>MASQPNSSAKKKEEKGKNIQVVVRCRPFNLAERKASAHSIVECDPVRKEVSVRTGGLADKSSRKTYTFDMVFGASTKQIDVYRSVVCPILDEVIMGYNCTIFAYGQTGTGKTFTMEGERSPNEEYTWEEDPLAGIIPRTLHQIFEKLTDNGTEFSVKVSLLSIYNEELFDLLNPSSDVSERLQMFDDPRNKRGVIIKGLEEITVHNKDEVYQILEKGAAKRTTAATLMNAYSSRSHSVFSVTIHMKETTIDGEELVKIGKLNLVDLAGSENIGRSGAVDKRAREAGNINQSLLTLGRVITALVERTPHVPYRESKLTRILQDSLGGRTRTSIIATISPASLNLEETLST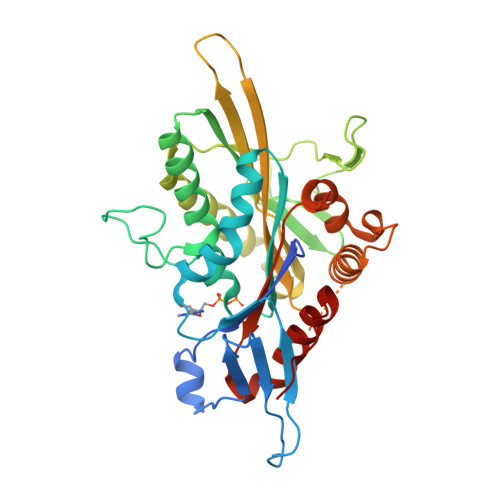LEYAHRAKNILNKPEVNQKL[2x]> GDRVADVIESSIGDSVSRALTQALPAPTGQNTQVSSHRLDTGEVPALQAAEIGASSNTSDESMIETRCVLNSHSTAETTLDSFFSRA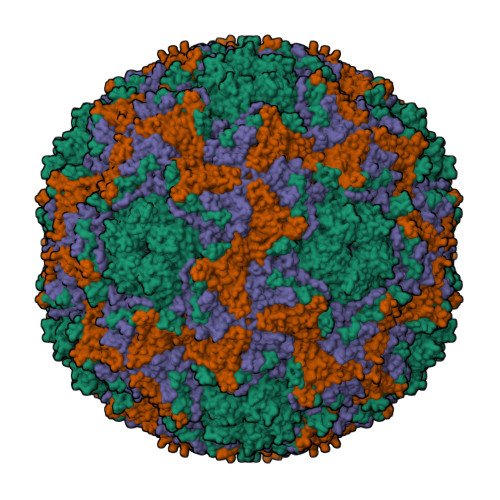GLVGEIDLPLEGTTNPNGYANWDIDITGYAQMRRKVELFTYMRFDAEFTFVACTPTGQVVPQLLQYMFVPPGAPKPESRESLAWQTATNPSVFVKLTDPPAQVSVPFMSPASAYQWFYDGYPTFGEHKQEKDLEYGACPNNMMGTFSVRTVGSSKSKYPLVVRIYMRMKHVRAWIPRPMRNQNYLFKANPNYAGNSIKPTGTSRSAITTL;> SPSAEACGYSDRVAQLTIGNSTITTQEAANIIVGYGEWPSYCSDDDATAVDKPTRPDVSVNRFYTLDTKLWEKSSKGWYWKFPDVLTETGVFGQNAQFHYLYRSGFCIHVQCNASKFHQGALLVAILPEYVIGTVAGGTGTEDSHPPYKQTQPGADGFELQHPYVLDAGIPISQLTVCHHQRINLRTNNCATIIVPYMNTLPFDSALNHCNFGLLVVPISPLDFDQGATPVIPITITLAPMCSEFAGLRQAVTQ;> GFPTELKPGTNQFLTTDDGVSAPILPNFHPTPCIHIPGEVRNLLELCQVETILEVNNVPTNATSLMERLRFPVSAQAGKGELCAVFRADPGRDGPWQSTMLGQLCGYYTQWSGSLEVTFMFTGSFMATGKMLIAYTPPGGPLPKDRATAMLGTHVIWDFGLQSSVTLVIPWISNTHYRAHARDGVFDYYTTGLVSIWYQTNYVVPIGAPNTAYIIALAAAQKNFTMKLCKDTSHILQTASIQ;> MGSQVSTQRSGSHENSNSATEGSTINYTTINYYKDSYAATAGKQSLKQDPDKFANPVKDIFTEMAAPLK>GPGVGESLPDLKIEKLDEGVYVHTSFEEVNGWGVVPKHGLVVLVNAEAYLIDTPFTAKDTEKLVTWFVERGYKIKGSISSHFHSDSTGGIEWLNSRSIPTYASELTNELLKKDGKVQATNSFSGVNYWLVKNKIEVFYPGPGHTPDNVVVWLPERKILFGGCFIKPYGLGNLGDANIEAWPKSAKLLKSKYGKAKLVV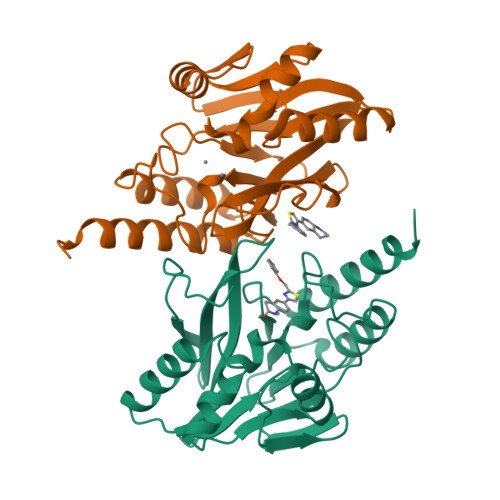PSHSEVGDASLLKLTLEQAVKGLNESKKPS[4x]>[4x]MSLDFNTLAQNFTQFYYNQFDTDRSQLGNLYRNESMLTFETSQLQGAKDIVEKLVSLPF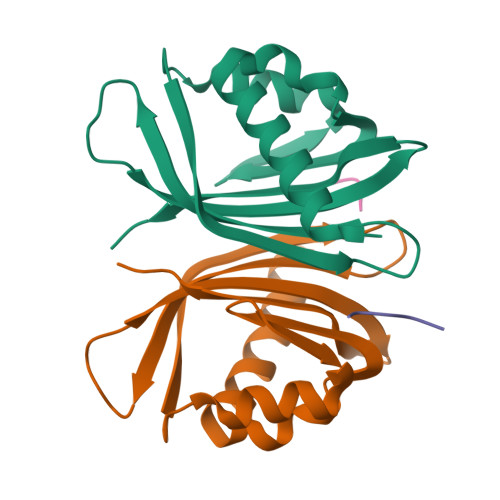QKVQHRITTLDAQPASPYGDVLVMITGDLLIDEEQNPQRFSQVFHLIPDGNSYYVFNDIFRLNYSA;>[4x]DSGFSFGSK> MLTSVLVRLVAWSVRRPIWVVVLSLVIAALSSVYVAHHFKINTDISKLVENDPKWAALGRAIDDAFPQRNQTILAVVEAPAPEFAGAAADALAEGLRRETEAGRIGQVSEPAGGPLFEHDGLLFLPEQDVATTTAQLASARPLINVLAKDPSIAGLATTLSTTLGVPLQSGQVKLSGMAKLLSRSAATVDDVLAGKPAAFSWRALVDADAAREPARAFVTVQPVVNYGALKAGEQASRTIRATAQALKLDERFGAAVRLTGEQPLADEEFASVQDGALVNGIATLAIVLVILWIALRSKRMIASVFVTL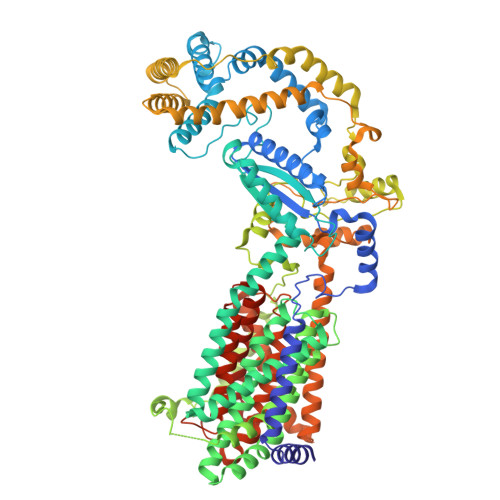FVGLVVTAALGLMMVGSLNMISVAFMVLFVGLGVDFAIQYGVKYREERHRDPNLDHALVGAAHAMGMPLTLATAAVAASFFSFLPTAYRGVSELGLIAGVGMFVALFTTLTLLPALLKLLAPPGERKPPGFPRLAPVDDYLDHHRKPILIGTLAVVIGALPLLAHLRFDFNPLHLKDPRSESMATLLALKDSPEASVNDVSLLAPSLVAANAAAQRLGALPEVGRTTTLSTFIPDAQPQKLATIAAAARGLLPALTQPAAAPVPDAQRVAALKRASNLLEYASEDYPGPGAAAAKHLSESLAKLAAADAATRERAEHAFSVPLKIALNQLAMLLQPLEITRENLPPQIVRDWIAPDGRALVQISPKVVKGADPGDDAMLRRFAKAVKAAEPGAIGGPISILHSADTIIRAFLQAAALSVVSITVLLWITLRRFGDVLRTLVPLLVSGVVTLELCVLLGMPLNFANIIALPLMLGVGVAFKVYFVMAWRAGQTGLLQSSLTHAVLFSAATTATAFGSLWLSHHPGTASMGRLLALALSCTLIGAVVFQPVLMGKPRTKRVTNQSQGIDE>MAEAAAAAAAAAAAGETSASSGSAAERDPDQDRAGRRLRVLSGHLLGRPQEALSTNECKARRAASAATAAPTATPAAPESGIIPKKRQELMKWNGWGYNDSKFFLNKKGQLELTGKRYPLSGVALPTFKDWIQNTFGINLDHKTTSKASLNPSDTPPSIVNEDFLHELKKTNISYSQEADDRVFRAHGHCLHEIFLLREGMFERIPDIVLWPTCHDDVVKIVNLACKYNLCIIPIGGGTSVSYGLMCPADETRTIISLDTSQMNRILWVDENNLTAHVEAGITGQELERQLKESGYCTGHEPDSLEFSTVGGWISTRASGMKKNIYGNIEDLVVHMKVVTPRGVIEKSCQGPRMSTGPDIHHFIMGSEGTLGVITEATIKIRPTPEYQKYGSVAFPNFEQGVACLREIAKQRCAPASIRLMDNQQFQFGHALKPQVSSIFTSFLDGLKKFYITKFKGFDPNQLSVATLLFEGDREKVLQHEKQVYDIAAKFGGLAAGEDNGQRGYLLTYVIAYMRDLGLEYYIIGESFETSAPWDRVVDLCRNVKERIRRECKEKGVQFPPLSTCRVTQTYDAGACIFFYFAFNYRGISDPLAVFEQTEAAAREEILANGGSLSHHHGVGKLRKQWLKESISDVGFGMLKSVKDYVDPTNIFGN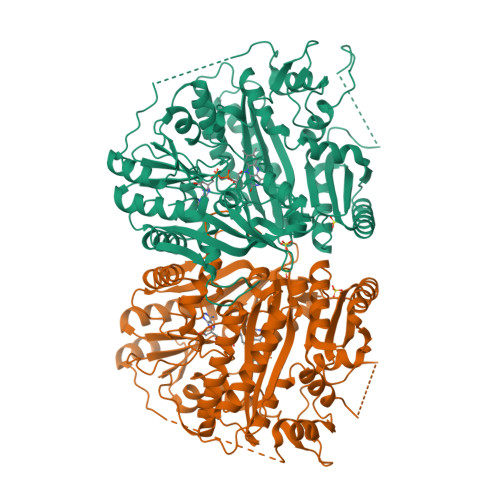RNLL[4x]> GPLGSPEFPGMSKVFIATANAGKAHDADIFSVSACNSFTVSCSGDGYLKVWDNKLLDNENPKDKSYSHFVHKSGLHHVDVLQAIERDAFELCLVATTSFSGDLLFYRITREDETKKVIFEKLDLLDSDMKKHSFWALKWGASNDRLLSHRLVATDVKGTTYIWKFHPFADESNSLTLNWSPTLELQGTVESPMTPSQFATSVDISERGLIATGFNNGTV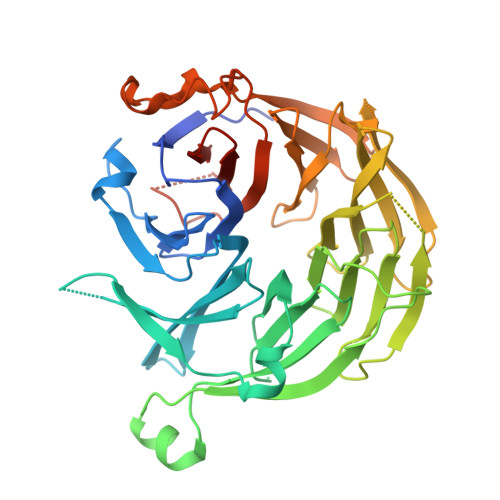QISELSTLRPLYNFESQHSMINNSNSIRSVKFSPQGSLLAIAHDSNSFGCITLYETEFGERIGSLSVPTHSSQASLGEFAHSSWVMSLSFNDSGETLCSAGWDGKLRFWDVKTKERITTLNMHCDDIEIEEDILAVDEHGDSLAEPGVFDVKFLKKGWRSGMGADLNESLCCVCLDRSIRWFREAGGK[(2~{R},3~{S},4~{S},5~{S})-5-(6-aminopurin-9-yl)-4-[(2~{S},3~{S},4~{S},5~{S})-5-[[[[(2~{R},3~{R},4~{S},5~{S})-5-(6-aminopurin-9-yl)-3,4-bis(oxidanyl)oxolan-2-yl]methoxy-oxidanyl-phosphoryl]oxy-oxidanyl-phosphoryl]oxymethyl]-3,4-bis(oxidanyl)oxolan-2-yl]oxy-3-oxidanyl-oxolan-2-yl]methyl 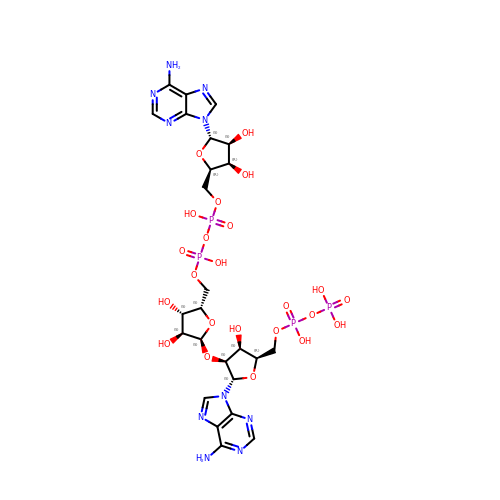phosphono hydrogen phosphate | C25 H36 N10 O23 P4 | CSEMRHUJDKFXPV-OATIKAJMSA-N>[2x]SKPQPIAAANWKCNGSESLLVPLIETLNAATFDHDVQCVVAPTFLHIPMT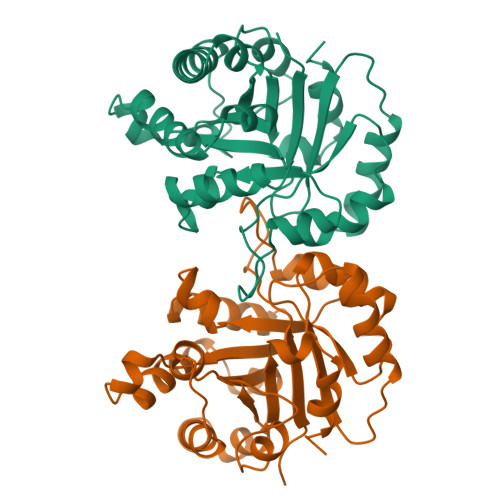KARLTNPKFQIAAQNAITRSGAFTGEVSLQILKDYGISWVVLGHSERRLYYGETNEIVAEKVAQACAAGFHVIVCVGETNEEREAGRTAAVVLTQLAAVAQKLSKEAWSRVVIAYEPVWAIGTGKVATPQQAQEVHELLRRWVRSKLGTDIAAQLRILYGGSVTAKNARTLYQMRDINGFLVGGASLKPEFVEIIEATK>[2x]MAEKPKLHYFNARGRMESTRWLLAAAGVE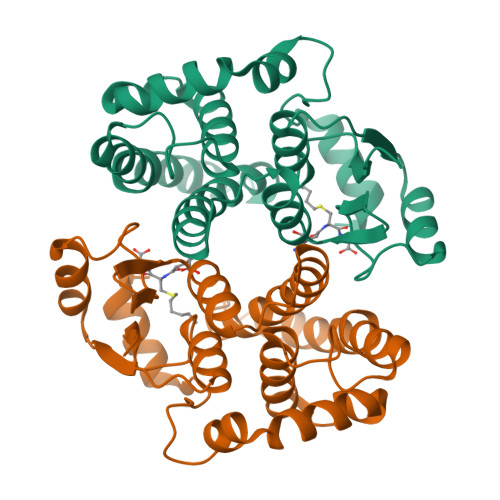FEEKFIKSAEDLDKLRNDGYLMFQQVPMVEIDGMKLVQTRAVLNYIASKYNLYGKDIKERALIDMYIEGIADLGEMILLLPVCPPEEKDAKLALIKEKIKNRYFPAFEKVLKSHGQDYLVGNKLSRADIHLVELLYYVEELDSSLISSFPLLKALKTRISNLPTVKKFLQPGSPRKPPMDEKSLEEARKIFRF> DNLIYL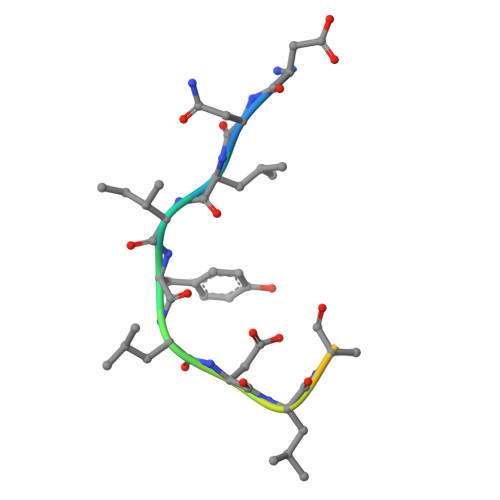DLNLQDWDD>[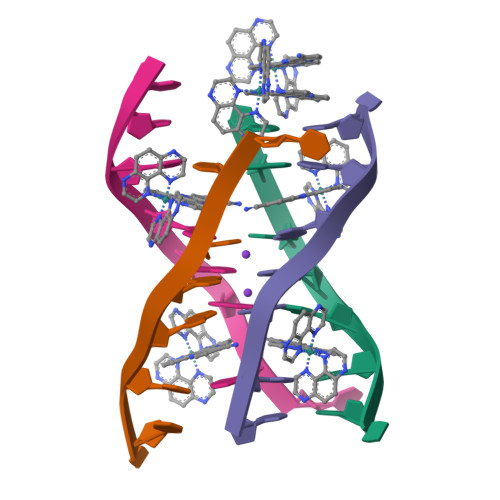4x]TAGGGTTA>QVVSQGWKYFKGNFYYFSLIPKTWYSAEQFCVSRNSHLTSVTSESEQEFLYKTAGGLIYWIGLTKAGMEGDWSWVDDTPFNKVQSARFWIPGEPNDAGNNEHCGNIKAPSLQAWNDAPCDITFLFICKRPYVPSEP[4x]

Langerin, a C-type lectin on Langerhans cells, mediates carbohydrate-dependent uptake of pathogens in the first step of antigen presentation to the adaptive immune system. The extracellular portion of langerin contains a C-type carbohydrate recognition domain (CRD)2 that binds sugars and a neck region that mediates formation of trimers stabilized by a coiled-coil of α-helices. As in other C-type lectins, the CRD of langerin contains a primary Ca2+-dependent sugar-binding site where Ca2+ forms direct coordination bonds with two vicinal hydroxyl groups of a monosaccharide. Langerin binds to a diverse set of glycan ligands including high mannose structures, β-glucans, and fucosylated blood group antigens.

To investigate the structural basis for the reduced binding of mannose-containing structures to the Asp-288/Ile-313 variant, the structure of this form of the CRD in complex with α-Me-Man was determined. The interactions of mannose with the principal Ca2+ through the 3- and 4-OH groups, as well as the additional interaction of the 2-OH group with the side chain of Lys-299, are the same as those observed for the wild type CRD. The Ile-313 side chain is distant from the mannose, consistent with the conclusion that this residue enhances binding to GlcNAc but plays little role in the affinity for mannose because the Asp-288 mutant alone shows a similar loss of affinity. Residue 288 is much closer to the principal Ca2+ site. The position of the side chain of Lys-257 remains the same in the presence of either aspartic acid or asparagine at position 288, and it does not have appropriate geometry to form hydrogen bonds with the side chain at position 288. However, the electrostatic interactions would be significantly different with aspartic acid at position 288 because this side chain forms a salt bridge with the amino group of Lys-257, which in turn forms part of a water-mediated hydrogen bond network with the side chain of Asp-308. Interactions with both backbone and side chain oxygen atoms of Asp-308 form a key part of the Ca2+-binding site. Thus, subtle differences in the hydrogen-bonding pattern resulting from the change of asparagine to aspartic acid at this position, could account for the reduced affinity for Ca2+, which in turn leads to an overall reduction in affinity for sugars. However, this form of langerin shows much weaker binding of the fucosylated blood group antigens and high mannose structures that are bound by wild type langerin and langerin-I313. Under the usual screening conditions of 2 mm CaCl2, the signals are lower, although the pattern of ligands bound is similar, with most significant binding to the GlcNAc-terminated ligands (data not shown). These results are consistent with previous experiments showing that the change of Asn-288 to aspartate results in a decrease in the affinity of the carbohydrate recognition domain for Ca2+ and thus a decrease in sugar binding affinity.> MSDLQQLFENNVRWAEAIKQEDPDFFAKLARQQTPEYLWIGCSDARVPANEIVGMLPGDLFVHRNVANVVLHTDLNCLSVIQFAVDVLKVKHILVTGHYGCGGVRASLHNDQLGLIDGWLRSIRDLAYEYREHLEQ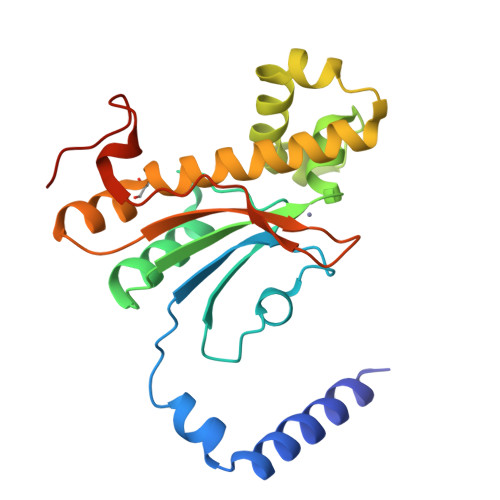LPTEEERVDRLCELNVIQQVANVSHTSIVQNAWHRGQSLSVHGCIYGIKDGLWKNLNVTVSGLDQLPPQYRLSPLGGCC>MAHHHHHHVDDDDKMTTSKLVVTPLGSLAFQYAEGIKGFNSQKGLFDVAIEGDSTATAFKLTSRLITNTLTQLDTSGSTLNVGVDYNGTAVEKTGDTVMIDTANGVLGGNLSPLANGYN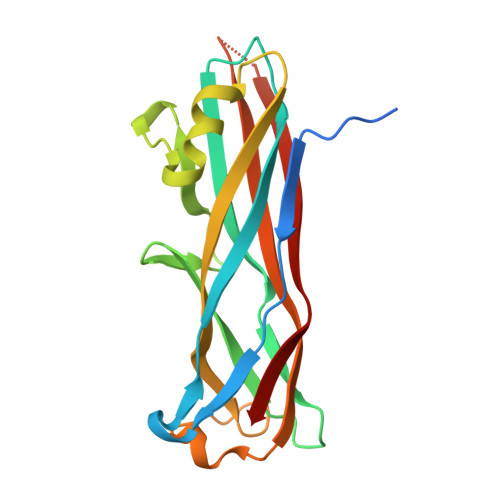ASNRTTAQDGFTFSIISGTTNGTTAVTDYSTLPEGIWSGDVSVQFDATWTSSDNKLRAAVSKTTWADAPARE[12x]>ALFALSLPVLAGPAVTPSSQIETDLLPASLLQISETEAFSRYVILVDKEQRKLSVFERNGEQIQKITEYPADIGKMGGNKTKRDDHKTPEGIYFLQERLSQPKIPFSLYGALAFTTNYPNLFDKRENKTGSGIWLHAIPDSVPLTRGSRGCVVVRNDVIKKLADYIKLGETPILIFDHVNYVSKSEHDKRRQDLSRFVESWRQAWENQDIEKYQTFYDEGFKAPGFNYKSWMSHKKNLKSKYEYIKVHLSQPYIVQHNDQLLVKTLQRYESDKHVDYGVKTIYALKSGDTYKIIREEWAPFSQQEVAAAIARENSMTASSQKTQ[2x]

Bdellovibrio bacteriovorus HD100 is a small, vibrioid-shaped predatory bacterium that invades and then replicates within the periplasm of Gram-negative prey bacteria, forming a spherical structure called a prey bdelloplast. The protein, Bd1075, generates cell curvature in B. bacteriovorus by exerting LD-carboxypeptidase activity upon the predator cell wall as it grows inside spherical prey. Bd1075 is targeted to the outer convex cell face by its C-terminal nuclear transport factor 2-like (NTF2) domain, where it exerts localized LD-carboxypeptidase (LD-CPase) activity upon the B. bacteriovorus PG wall to generate curvature and the classical vibrio shape.

The structure of mature Bd1075 protein was determined to 1.34 Å. The Bd1075 structure contains two domains: the catalytic LD-CPase domain (aa 47–180) and a C-terminal nuclear transport factor 2 (NTF2)-like domain (aa 196–304). Interestingly, although there was a global agreement in the fold to Csd6 of H. pylori and Pgp2 of C. jejuni which also contain an NTF2 domain and an LD-CPase domain (the junction between the two at residue 188 of Bd1075), there were significant differences in fold elements and local regions. These differences resulted in an inability to solve Bd1075 via molecular replacement, necessitating the use of SAD phasing with co-crystallized halide ions. We were able to trace residues 29–308 with the exception of a presumably flexible region (aa 82–91) which we term the active site ‘lid’. Bd1075 has a consensus active site, with the superfamily conserved catalytic triad consisting of C156, H141, and A142, each present in the expected (presumed active) orientations. The termini of Bd1075 are very different to both Csd6 and Pgp2, replacing the N-terminal dimerization domain of those enzymes with a simple, shorter loop, and extending the C-terminus such that the Bd1075 NTF2 domain finishes with a longer beta-strand (aa 295–306)—residues of which contribute to its binding pocket. Most noteworthy within the core of the Bd1075 C-terminus was the presence of W303, which is clearly located within the substrate-binding pocket of the NTF2 domain. The crystal packing of Bd1075 was such that a two amino acid loop of P107/K108 from one Bd1075 monomer packed into the NTF2 domain of the adjacent monomer. We postulate that its position has been modified in our Bd1075 structure by sidechains contacting the P107/K108 loop and may thus represent a ‘bound’ state.> MRRAVGVPPVMAYAEGPPPSYESVMGSADSPATLEALYVPPRYLGPTEGRNSIRYSELAPLYDTTRVYLVDNKSADIASLNYQNDHSNFQTTVVQNNDFTPAEAGTQTINFDERSRWGADLKTILRTNMPNINEFMSTNKFKARLMVEKKNKETGLPRYEWFEFTLPEGNYSETMTIDLMNNAIVDNYLEVGRQNGVLESDIGVKFDTRNFRLGWDPVTKLVMPGVYTNEAFHPDIVLLPGCGVDFTQSRLSNLLGIRKRLPFQEGFQIMYEDLEGGNIPALLDVAKYEASIQKAKEEGKEIGDDTFATRPQDLVIEPVAKDSKNRSYNLLPNDQNNTAYRSWFLAYNYGDPKKGVQSWTLLTTADVTCGSQQVYWSLPDMMQDPVTFRPSTQVSNYPVVGVELLPVHAKSFYNEQAVY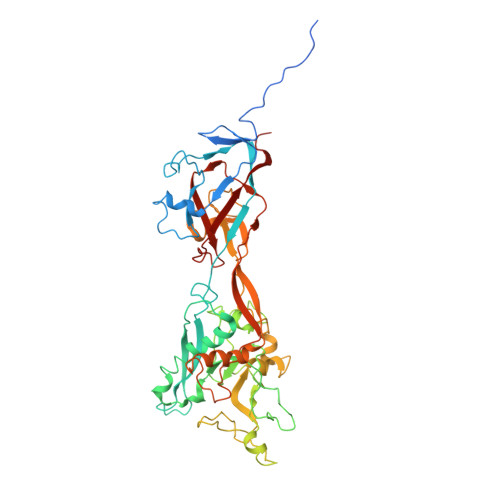SQLIRQSTALTHVFNRFPENQILVRPPAPTITTVSENVPALTDHGTLPLRSSISGVQRVTITDARRRTCPYVHKALGIVAPKVLSSRTF> MLYKELGRTGEEIPALGLGTWGIGGFETPDYSRDEEMVELLKTAIKMGYTHIDTAEYYGGGHTEELIGKAIKDFRREDLFIVSKVWPTHLRRDDLLRSLENTLKRLDTDYVDLYLIHWPNPEIPLEETLSAMAEGVRQGLIRYIGVSNFDRRLLEEAISKSQEPIVCDQVKYNIEDRDPERDGLLEFCQKNGVTLVAYSPLRRTLLSEK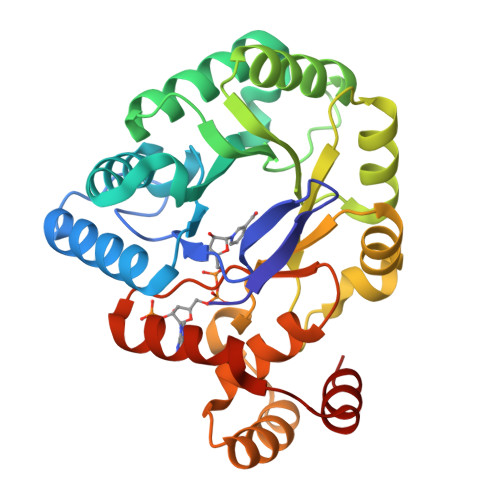TKRTLEEIAKNHGATIYQIMLAWLLAKPNVVAIPKAGRVEHLRENLKATEIKLSEEEMKLLDSLG>SHMEDYIEAIANVLEKTPSISDVKDIIARELGQVLEFEIDLY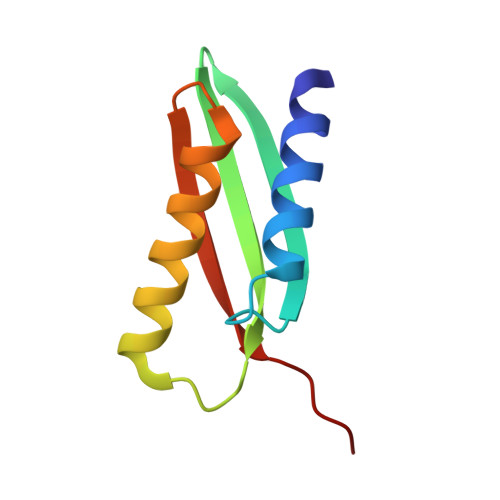VPPDITVTTGERIKKEVNQIIKEIVDRKSTVKVRLFAAQEEL[6x]>MHHHHHHSSGRENLYFQGVDLELRVLEESDLSSHLELLGHLTEAPPLSGVELANIADMRRRAGIVTKVFCHQ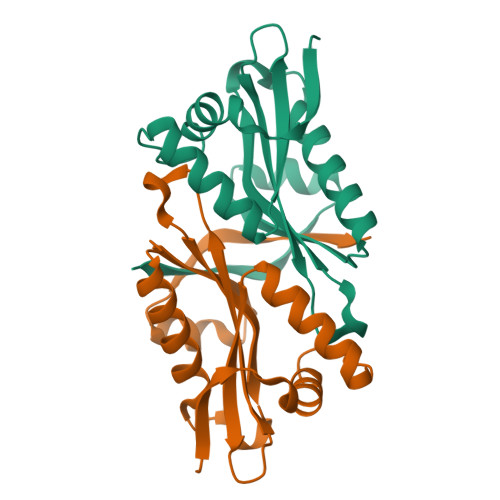PTGRIVGSASLMIQPKFTRGGRAVGHIEDVVVDPSYRGAGLGKALIMDLCEISRSKGCYKVILDSSEKSLPFYEKLGFRAHERQMRLDL[2x]Rab11 family-interacting protein 2 (FIP2) is a 512-residue effector that contains a Rab-binding domain (RBD) at its C-terminus. The effector FIP2 contains an N-terminal C2 domain that binds to phospholipids (residues 15–102; Lindsay & McCaffrey, 2004), a myosin Vb-binding domain (residues 129–290; Hales et al., 2002) and a C-terminal RBD (residues 440–512; Hales et al., 2001) that binds to Rab11. The N-terminus of this modular effector family is variable and consists of domains that include EF-hands, ERM domains, C2 domains and myosin V-binding domains. These effectors regulate membrane trafficking following their recruitment to subcellular compartments by Rab11, Rab14 and Rab25 GTPases. The crystal structures of Rab11–FIP2, Rab11–FIP3 and Rab25–FIP2 complexes revealed that the RBD is a parallel α-helical coiled coil.

Here, the crystal structure of an uncomplexed form of FIP2 was determined at 2.3 Å resolution by the ab initio phasing method in ARCIMBOLDO. In contrast to previous crystal structures of complexes, the structure of isolated FIP2 reveals the formation of antiparallel α-helical dimers that are stabilized by polar interactions. Although the segment 439–512 was subjected to crystallization, a minimum of the first seven residues and the last 15 residues are dis­ordered. The polypeptides are of varying lengths depending on the extent of disorder at the N/C-termini. The structure reveals antiparallel α-helices that associate through polar interactions. These include a remarkable stack of arginine residues within a four-helix bundle in the crystal lattice. The distances between the Cζ atoms in the stacked guanidino side chains are 3.5–3.8 Å. Aspartate residues form salt bridges with these arginines and presumably contribute to orienting the guanidino groups (not shown). Since crystal formation required the presence of a small amount of Co2+, data were also collected at the Co2+ absorption edge. Also, FIP2 spontaneously forms dimers in solution at physiological pH. It is probable that parallel dimers dissociate to form the crystals observed here at pH 4.8. Therefore, the physiological relevance of the structure of uncomplexed FIP2 observed under these conditions is unknown.

>[4x]GSHMSNPFDATAGYRSLTYEEVLQELVKHKELLRRKDTHIRELEDYIDNLLVRVMEETPSILRVPYEPSRKAGKFSNS>[2x]SPSINVALKAAFPSPPYLVELLETAASDNTTIYYSLLDRIAKGHFAEATTDKALYEKFLEVLRDDGHMDPEALSAFKLALSLRTATPRVEAHYQYYTATVEPSLSGTQEGCDQWFLIDGEQYCSPTLDTSHGKVKGEDQLRTLPFDRKFCVGSRDVILYADITSKSFAPFHEVAMDLAKKGKASYRVRYRRSPSHSRESLSVNGYGVELVLKRTDYIVIDDRDTGAAAKPAEENDQKPLVGHETVLDDGEEIADIKPLEKSELAALGMKAASFVMQSEKPFEALLKLTQDFPKYSNSLGSQNVSAEFEAEHRGNREVFLPEGSNVLWLNGLHLIDRQIQPFGLVDLLTRERKLIKSVLDLGLTGQQAVDLLGHAEVAHAKSGDDEPRRFDWRDDIEEGQVIIWLNNLEKDKRYKSFSPSIWVLIHHFGHGLPQIRRDVFNLVVPVDLTKADDVKIVVEGLLSFVKRLIPVRFGFVPLTPTGQAIDQAKVVYYLLENYGLAAATAYLEKSYEEQSTGQPNERIFNEVIKDKSLRPDGVELSFKDIFISEKHEKQIHLSKHWVERLRAGGDVPTVFFDGFPIPRE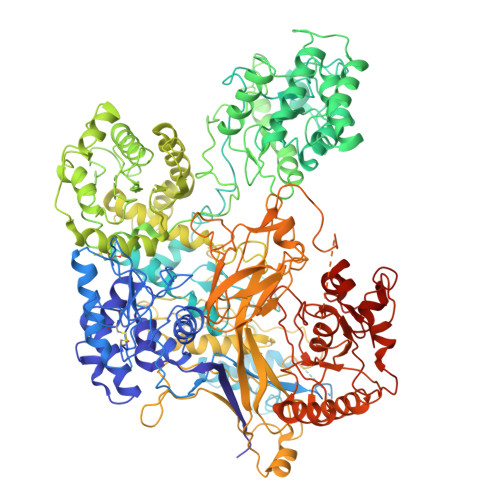DNWLRVMNHRLMQDLQALQQAGYFGMLNESMWLPGFFLEKALSRRNTLIFPEDKNELTVLNVNKIYIENHDLMSKVPVIEASKESTRDDWAALTVVADLDDIEGQELVYYALRFRKSNDGVRLDIVHNPKDTSRSPSVLAQRLKSREDKLLDFTRFLDLETALETGEFEPDVAYDCSLANFLASSNMKAGDNFVILNGRVLGPITSADDFKKEDFEVFLQAERRTRILPVYKALEDLGLDDKVSGPLSAAKLTSVTALSTISDLPQGIFDNAPTVRTTLFKQWNSTYTSFEVGDASTATIFFVAVINPASEIGQRWVAVLKVLSELEGVHLRVFLNPTVMIEELPVKRFYRYVLSSSPSFDESGKVKALSARFTGVPRETLLVVGMDVPPAWLVTSKVAVDDLDNLRIKDIKAKRGTEHVEAIYELEHILIEGHSREIPGAHAPRGVQLVLETENNPHFADTIIMANLGYFQFKANPGVYNIRLKEGRSSEIFTLESVGAKGWGPIPGDDNTEVVLMDFQGTTLYPRLRRKPGMEEEDVLEPSTKSGEESGSGARNLVSRGIKFAEGLLGRGNKAAEATKSVSKTEHAEINIFSVASGHLYERMLNIMMASVMHHTNHTVKFWFIEQFLSPSFKDFIPHMAAEYGFKYEMVTYKWPHWLRQQKEKQREIWGYKILFLDVLFPLSLDKVIFVDADQIVRTDMYDLVEHPLDGAPYGFAPMCDSRVEMEGYRFWKTGYWANYLKGKPYHISALYVVDLQRFRELAAGDRLRQQYHALSADPNSLANLDQDLPNHMQFTIPI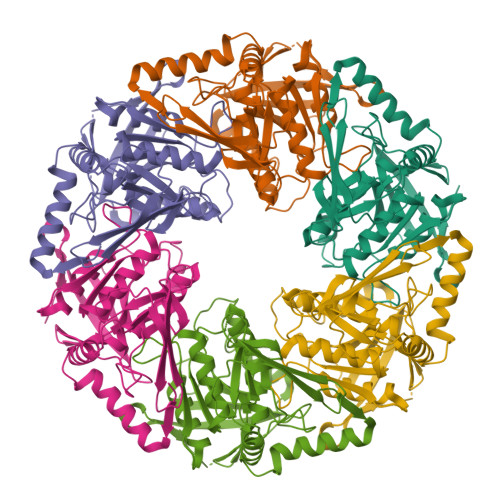>[24x]MIHLYDAKSFAKLRAAQYAAFHTDAPGSWFDHTSGVLESVEDGTPVLAIGVESGDAIVFDKNAQRIVAYKEKSVKAEDGSVSVVQVENGFMKQGHRGWLVDLTGELVGCSPVVAEFGGHRYASGMVIVTGKGNSGKTPLVHALGEALGGKDKYATVRFGEPLSGYNTDFNVFVDDIARAMLQHRVIVIDSLKNVIGAAGGNTTSGGISRGAFDLLSDIGAMAASRGCVVIASLNPTSNDDKIVELVKEASRSNSTSLVISTDVDGEWQVLTRTGEGLQRLTHTLQTSYGEHSVLTIHTSKQSGGKQASGKAIQTVIKNDELESVLRRLTSN> MIPQTLTNTNLFIDGVSFAGDVPSLTLPKLAVKTEQYRAGGMDAPVSIDMGLEAMEAKFSTNGARREALNFFGLADQSAFNGVFRGSFKGQKGASVPVVATLRGLLKEVDPGDWKAGEKAEFKYAVAV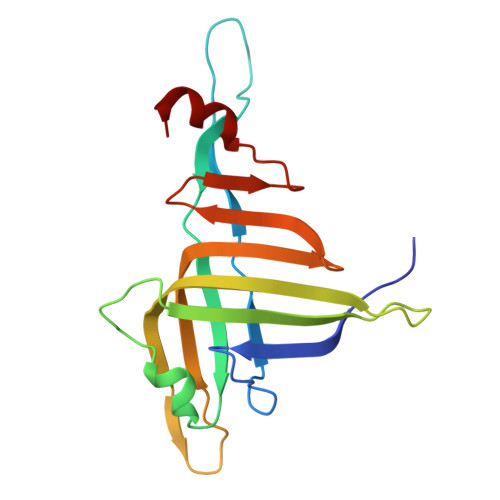SYYKLEVDGREVYEIDPVNGVRAINGVDQLAGMRNDLGL> GKRRVSYFYEPMIGDYYYGVNQPTKPQRIRVTHNLILSYNLHRHMEINHPDLADASDFEKFHSLEYINFLKSVTPETVTDPHPSVSENLKRFNVDVDWDGPVFHNLFDYCRAYAGGSISAAAKLNRQEADIAINWAGGMHHVKKDKASGFGYVNDVVLAILELLKSFKRVLYIEIGFPHGDEVEEA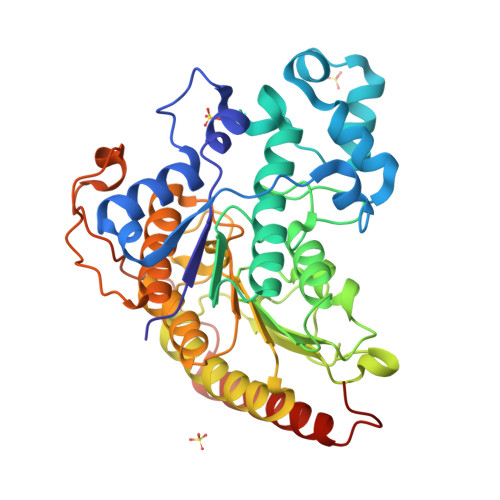FKDTDRVMTVSFHKVGDTGDISDYGEGKGQYYSLNAPLKDGLDDFSLRGLFIPVIHRAMEIYEPEVIVLQCGADSLAGDPFGTFNLSIKGHGDCLQYVRSFNVPLMILGGGGYTLPNVARCWCYETAIAVGEQLDNDLPGNDYMKYFRPDYKLHILPTNRQNLNTRLDIITMRETLLAQLSLVMHAPSVPLEHHHHHH>[2x]XSEPIRVLVTGAAGQIAYSLLYSIGNGSVFGKDQPIILVLLDITPMMGVLDGVLMELQDCALPLLKDVIATDKEEIAFKDLDVAILVGSMPRRDGMERKDLLKANVKIFKCQGAALDKYAKKSVKVIVVG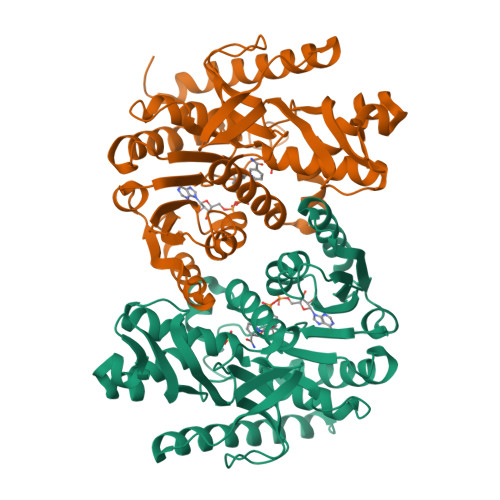NPANTNCLTASKSAPSIPKENFSCLTRLDHNRAKAQIALKLGVTSDDVKNVIIWGNHSSTQYPDVNHAKVKLQAKEVGVYEAVKDDSWLKGEFITTVQQRGAAVIKARKLSSAMSAAKAICDHVRDIWFGTPEGEFVSMGIISDGNSYGVPDDLLYSFPVTIKDKTWKIVEGLPINDFSREKMDLTAKELAEEKETAFEFLSSA> MRGSHHHHHHGSAPAQAANPYERGPNPTESMLEARSGPFSVSEERASRFGADGFGGGTIYYPRENNTYGAIAISPGYTGTQSSIAWLGERIASHGFVVIAIDTNTTLDQPDSRARQLNAALDYMLTDASSAVRNRIDASRLAVMGHSMGGGGTLRLASQRPDLKAAIPLTPWHLNKSWRDIT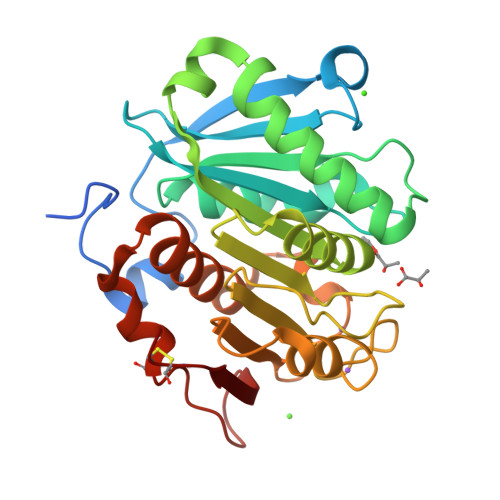VPTLIIGAEYDTIASVTLHSKPFYNSIPSPTDKAYLELDGASHFAPNITNKTIGMYSVAWLKRFVDEDTRYTQFLCPGPRTGLLSDVEEYRSTCPF>GARASVLSGGELDKWEKIRLRPGGKKQYKLKHIVWASRELERFAVNPGLLETSEGCRQILGQLQPSLQTGSEELR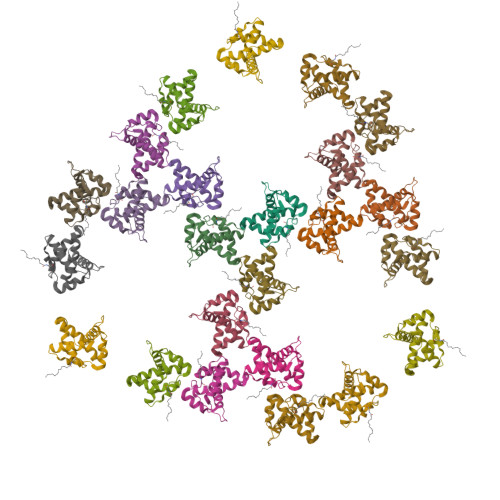SLYNTIAVLYCVHQRIDVKDTKEALDKIEEEQNKSKKKAQ[24x]>[2x]AAPDEITTAWPVNVGPLNPHLYTPNQMFAQSMVYEPLVKYQADGSVIPWLAKSWT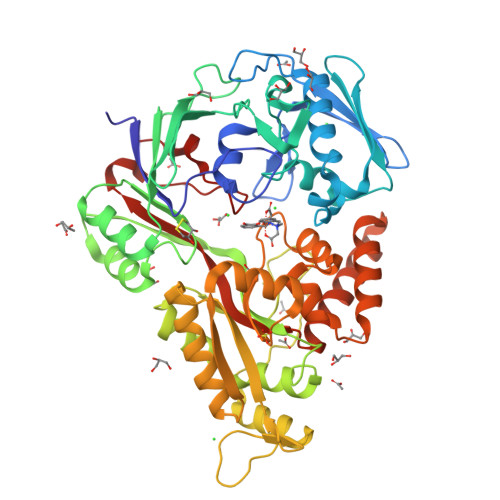HSEDGKTWTFTLRDDVKFSNGEPFDAEAAAENFRAVLDNRQRHAWLELANQIVDVKALSKTELQITLKSAYYPFLQELALPRPFRFIAPSQFKNHETMNGIKAPIGTGPWILQESKLNQYDVFVRNENYWGEKPAIKKITFNVIPDPTTRAVAFETGDIDLLYGNEGLLPLDTFARFSQNPAYHTQLSQPIETVMLALNTAKAPTNELAVREALNYAVNKKSLIDNALYGTQQVADTLFAPSVPYANLGLKPSQYDPQKAKALLEKAGWTLPAGKDIREKNGQPLRIELSFIGTDALSKSMAEIIQADMRQIGADVSLIGEEESSIYARQRDGRFGMIFHRTWGAPYDPHAFLSSMRVPSHADFQAQQGLADKPLIDKEIGEVLATHDETQRQALYRDILTRLHDEAVYLPISYISMMVVSKPELGNIPYAPIATEIPFEQIKPVK> MAVEVLKEKWNSKVVEVTLGTGDKTVTLGGDSTLPFLTFEGEMPNPPRFALEVFDTPPTDWPDILVEPFKDVINDPVAWAKKCVEYGADIVALRLVSAHPDGQNRSGAELAEVCKAVADAIDVPLMIIGCGVEEKDAEIFPVIGEALSGRNCLLSSATKDNYKPIVATCMVHGHSVVASAPLDINLSKQLNIMIMEMNLAPNRIIMDPLIGALGYGIEY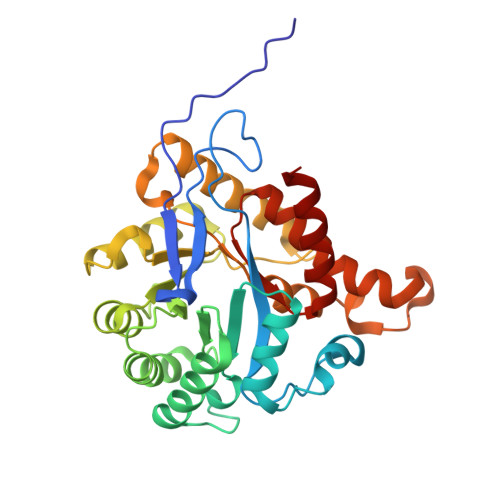SYSIIERMRLGALTGDKILAMPVVCFIGQEAWKAKEAKDPEVAEWGDYALRAIHWETVTTVALIQAGGHLFVMRHPKSLAEVKEHLKRILK>[7x]MAEQKSSNGGGGGGDVVINVPVEEASRRSKEMASPESEKGVPFSKSPSPEISKLVGSPNKPPRAPNQNNVGLTQRKSFARSVYSKPKSRFVDPSCPVDTSILEEEVREQLGAGFSFSRASPNNKSNRSVGSPAPVTPSKVVVEKDEDEEIYKKVKLNREMRSKISTLALIESAFFVVILSALVASLTINVLKHHTFWGLEVWKWCVLVMVIFSGMLVTNWFMRLIVFLIETNFLLRRKVLYFVHGLKKSVQVFIWLCLILVAWILLFNHDVKRSPAATKVLKCITRTLISILTGAFFWLVK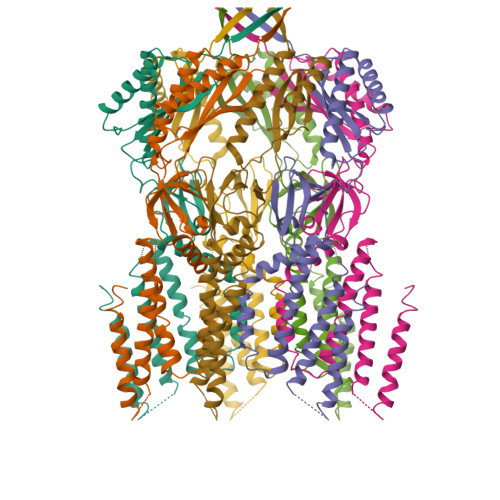TLLLKILAANFNVNNFFDRIQDSVFHQYVLQTLSGLPLMEEAERVGREPSTGHLSFATVVKKGTVKEKKVIDMGKVHKMKREKVSAWTMRVLMEAVRTSGLSTISDTLDETAYGEGKEQADREITSEMEALAAAYHVFRNVAQPFFNYIEEEDLLRFMIKEEVDLVFPLFDGAAETGRITRKAFTEWVVKVYTSRRALAHSLNDTKTAVKQLNKLVTAILMVVTVVIWLLLLEVATTKVLLFFSTQLVALAFIIGSTCKNLFESIVFVFVMHPYDVGDRCVVDGVAMLVEEMNLLTTVFLKLNNEKVYYPNAVLATKPISNYFRSPNMGETVEFSISFSTPVSKIAHLKERIAEYLEQNPQHWAPVHSVVVKEIENMNKLKMALYSDHTITFQENRERNLRRTELSLAIKRMLEDLHIDYTLLPQDINLTKKN>[2x]SGGKLTAVDPETNMNVSEIISYWGFPSEEYLVETEDGYILCLNRIPHGRKQHSDKGPKPVVFLQHGLLADSSNWVTNLAQSSLGFILADAGFDVWMGNSRGNTWSRKHKTLSVSQDEFWAFSYDEMAKYDLPASINFILNKTGQEQVYYVGHSQGTTIGFIAFSQIPELAKRIKMFFALGPVASVAFCTSPMAKLGRLPDHLIKDLFGDKEFLPQSAFLKWLGTHVCTHVILKELCGNLCFLLCGFNERNLNMSRVDVYTTHSPAGTSVQNMLHWSQAVKFQKFQAFDWGSSAKNYFHYQQSYPPTYNVKDMLVPTAVWSGGHDWLADVYDVNILLTQITNLVFHESIPEWEHLDFIWGLDAPWRLYNKIINLMRKYQASENNL

Lysosomal acid lipase (LAL) is a serine hydrolase enzyme located in the lysosome, where it breaks down cholesteryl esters (CEs) and TGs into free cholesterol and fatty acids (1–3). LAL belongs to a gene family of mammalian acid lipases that includes gastric and lingual lipases. Unlike the well-known mammalian lipases of the lipase superfamily, triacylglycerol lipases, LAL shows a dual catalytic activity, capable of hydrolyzing both TG and CE. LAL deficiency in humans results in multisystem autosomal recessive disease phenotypes, WD and CESD.

In the present study, we have expressed and purified a triple glycosylation mutant (TGM) (N51Q, N80Q, and N300Q; mature protein numbering) of HLAL and determined the crystal structure at 2.6 Å resolution in its lid-closed conformation. The recombinant HLAL-TGM was crystallized in the orthorhombic space group P21212 with two molecules in the asymmetric unit and diffracted to around 2.6 Å. The overall architecture consists of a core domain and a cap domain. The core domain, which constitutes residues 9–183 and 310–384 (mature protein numbering), contains a central β-sheet composed of eight strands (seven parallel) and six helices, three on each side of the β-sheet. The cap domain fold (residues 184–309) is a complex mixture of eight helices, turns, and random coils, including a lid (residues 215–244) that adapts a “closed” conformation. The structure also includes GlcNAC sugar residues on three of the N-glycosylation sites (Asn-15, Asn-140, and Asn-252); the other three potential sites (Asn-51, Asn-80, and Asn-300) were mutated to Gln. Among these, Cys-227 and Cys-236 (mature protein numbering) form a disulfide bridge (Cys-227–Cys-236), whereas the other Cys residues are free, as previously discussed in the case of HGL. As suggested before, Pro-241 and Gly-245 residues flank the lid acting as hinges, with the trans-cis-proline isomerization inducing opening and closing of the lid. It is apparent from the structure that the catalytic Ser-153 is completely inaccessible and substantial conformational changes must take place before substrate can bind in the postulated active site. Cys-240 and Cys-244 are in the lid region and are deeply buried pointing toward the catalytic Ser-153 (Cys-244 is only 5 Å away from catalytic Ser-153). In our HLAL structure, His-274 in the α13 helix is involved in a hydrogen bond interaction with Ser-122 and Gln-285, is sandwiched by two aromatic residues (Tyr-123 and Phe-287), and stabilizes the interaction between the α13 helix and a long loop-helix-loop region (residues 286–304).> ARGRG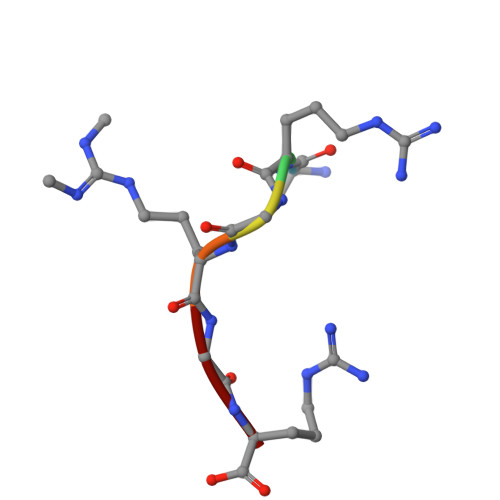R> ITSIWTKGVTPPTNFIEGTDGSHAPYIANQGWYDITKTFNGKDDLLSAAATAGNMLHWWFDQNKNQIEGYLTEHPEKQAIIFNGEQMFDVKEAISTKDRQLDSKLFEYFKEKAFPTLSARRRGVFPDHVIDMFINGYRLSLDNYDKTPVKEGNKDLRGGIFDQVFTRGDQSKLLTNRYNLRTKT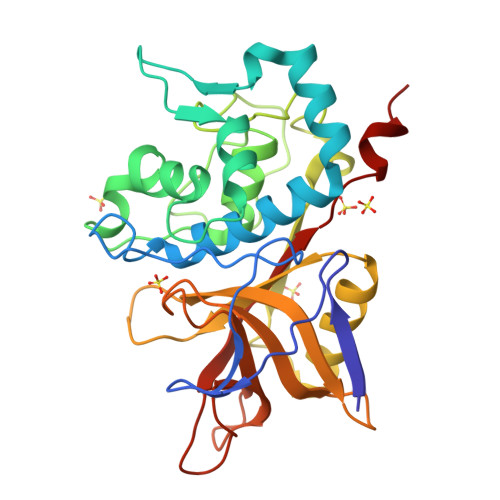INEISQLIKQELIAGKALAISHTYNNIGISHVINLWGADFNSEGNLEAIYVTDSDSNASIGMKKYYVGVNSAGEVAVSSKKIDSEHLGAAALGLYTLSAGQGIWHQTN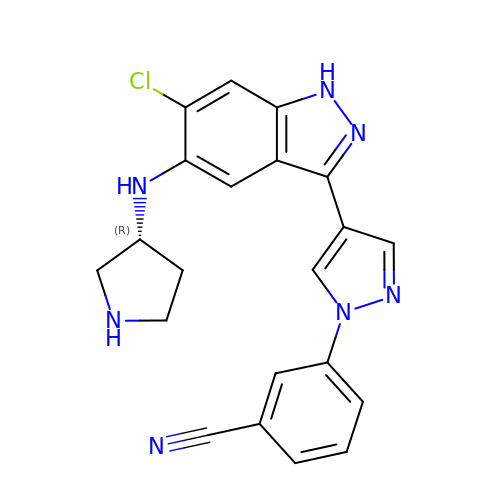3-[4-[6-chloranyl-5-[[(3R)-pyrrolidin-3-yl]amino]-1H-indazol-3-yl]pyrazol-1-yl]benzenecarbonitrile | C21 H18 Cl N7 | GLHJKYCHVYCTAN-OAHLLOKOSA-N>AYAQWVIIIIHNVGSKDVKIKNLKPSWGKLHADGDKDTEVSASKYEGTVIKPDEKLQINACGRSDAAEGTTGTFDLVDPADGDKQVRHFYWDCPWGSKTNTWTVSGSNTKWMIEYSGQNLDSGALGTITVDTLKK[2x];> SQAGDTLNDVIQDPTRRNKLINDNNLLKGIIMGRDGPVPSSRELIVRPDTLRAIINNRATIETTTMKSMYTSSRYLFPQGRIDFTTPDSGFDDVIKLSPQFTSGVQAALAKAT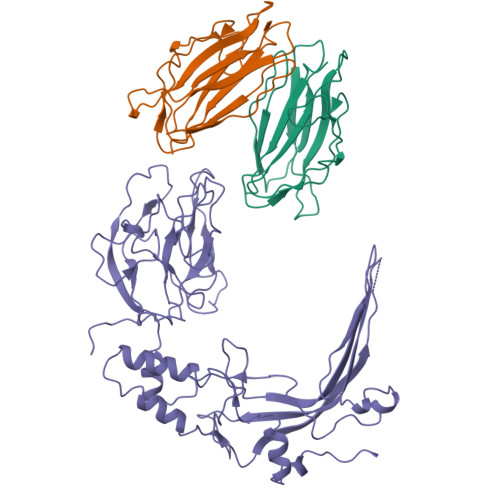GTEKREALQNLFQEYGHVFRTKVHIGGVLSAHTMETFSKLNVKYIVNGGDYTKIQNTEEWVASTNQSEHWRVIEVTEVTAVADLLPQPIRGQVKDLLKPLLGKWVDVEKVPGLESLPVSVYRPKGAIPAGWFWLGDTADASKALLVKPTLPARSGRNPALTSLHQGSGMTEQPFVDLPQYQYLSTYFGSFAHDTPPGSTLRGLRPDHVLPGRYEMHGDTISTAVYVTRPVDVPFPEDECFDLKSLVRVKLPGSGNPPKPRSALKKSMVLFDSGEK>[4x]K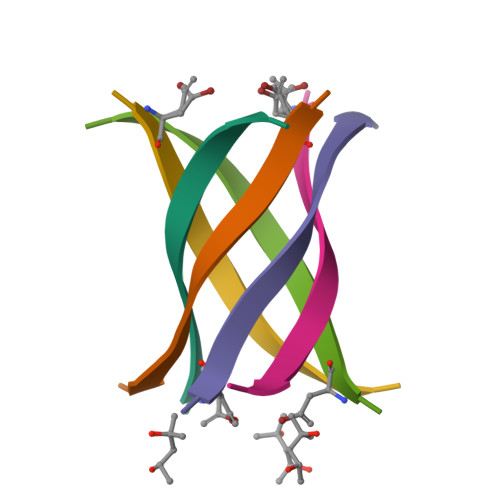XKVLGDVIEV> MATEHPEPPKAELQLPPPPPPGHYGAWAAQELQAKLAEIGAPIQGNREELVERLQSYTRQTGIVLNRPVLRGEDGDKAAPPPMSAQLPGIPMPPPPLGLPPLQPPPPPPPPPPGLGLGFPMAHPPNLGPPPPLRV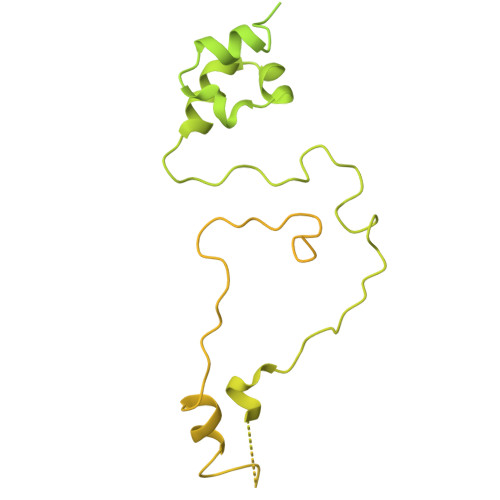GEPVALSEEERLKLAQQQAALLMQQEERAKQQGDHSLKEHELLEQQKRAAVLLEQERQQEIAKMGTPVPRPPQDMGQIGVRTPLGPRVAAPVGPVGPTPTVLPMGAPVPRPRGPPPPPGDENREMDDPSVGPKIPQALEKILQLKESRQEEMNSQQEEEEMETDARSSLGQSASETEEDTVSVSKKEKNRKRRNRKKKKKPQRVRGVSSESSGDREKDSTRSRGSDSPAADVEIEYVTEEPEIYEPNFIFFKRIFEAFKLTDDVKKEKEKEPEKLDKLENSAAPKKKGFEEEHKDSDDDSSDDEQEKKPEAPKLSKKKLRRMNRFTVAELKQLVARPDVVEMHDVTAQDPKLLVHLKATRNSVPVPRHWCFKRKYLQGKRGIEKPPFELPDFIKRTGIQEMREALQEKEEQKTMKSKMREKVRPKMGKIDIDYQKLHDAFFKWQTKPKLTIHGDLYYEGKEFETRLKEKKPGDLSDELRISLGMPVGPNAHKVPPPWLIAMQRYGPPPSYPNLKIPGLNSPIPESCSFGYHAGGWGKPPVDETGKPLYGDVFGTNAAEFQTKTEEEEIDRTPWGELEPSDEESSEEEEEEESDEDKPDETGFITPADSGLITPGGFSSVPAGMETPELIELRKKKIEEAMDGSETPQLFTVLPEKRTATVGGAMMGSTHIYDMSTVMSRKGPAPELQGVEVALAPEELELDPMAMTQKYEEHVREQQAQVEKEDFSDMVAEHAAKQKQKKRKAQPQDSRGGSKKYKEFKF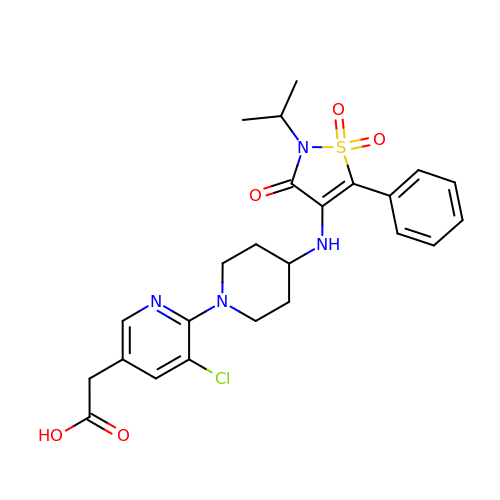2-[5-chloranyl-6-[4-[[1,1,3-tris(oxidanylidene)-5-phenyl-2-propan-2-yl-1,2-thiazol-4-yl]amino]piperidin-1-yl]pyridin-3-yl]ethanoic acid | C24 H27 Cl N4 O5 S | JSAUQHYJLCPNIF-UHFFFAOYSA-N> AATQQEIGKNMWDPFQSMRAVTGLMELTSGQCTQLSKDAAAILAGVKESHDSISVDKNYKVLNDEVAYHAANIDA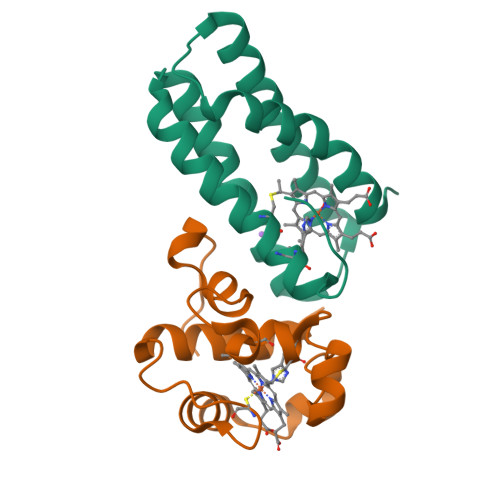AAKANDLEEVQVQFRRMTIACRNCHKIYKTEQRLVP;> LNEHTAGDTTKSPYTIYAGLGFAVQESCYYCHGNGGKGTTEGLIFGVPDFTSTEFQSSMTDKQIIDHINKGKGKCPSYQGKMSPEMIEKMAGVVRNFAVK> MGNKQV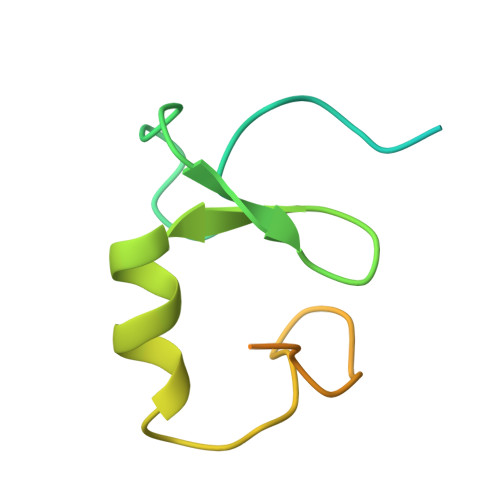KAPEARNSPRASLIPDATHLGPQFCKSCWFENKGLVECNNHYLCLNCLTLLLGVSSRCPICKMPLPTRLRPSAAPTAPPAEAGDNTRPPPYSP> AMPFEIEVLLPGELSPAETSALQKCEGKIITFSTLRHRASLVDIALSSYYINGAPPDT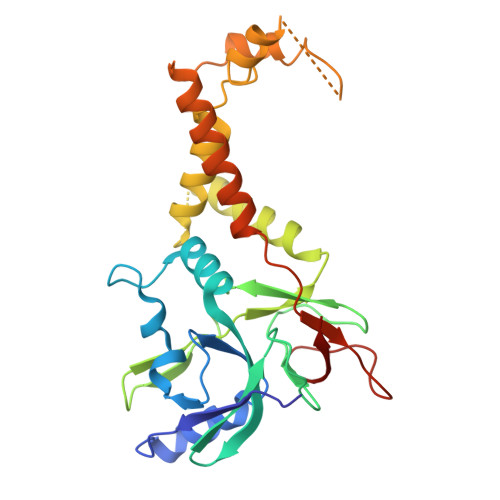LSLLEAYRMRFAAVITRVIPGKLLAHAIGVGTPTPGLFIQNTSPVDLCNGDYICLLPPVYGSADSIRLDSVGLEIVFPLTIPQTLMREIIAKVVARAVEDLNLMFSINEGCLLILALIPRLLALLIPRLLALVTREAAQLIHPEAPMLMLPIYETISSWISTSSRLGDTLGTRAILRVCVFDGPSTVHPGDRTAVIQV The Nef protein is an accessory gene product of HIV and SIV that is dispensable for virus spread in experimental ex vivo cell culture systems. Thus, Nef is an important factor for AIDS pathogenesis. To achieve this multitude of activities, Nef has evolved as versatile adaptor for protein interactions that lacks intrinsic enzymatic activity, which allows the viral protein to affect a wide range of host cell protein sorting and signal transduction processes. We thus chose a strategy aimed at wrapping the surface of Nef by the combination of different, physically linked, target domains and the iterative optimization of domain composition and linker segments.

Mutation of the RT-loop sequence E88AIHHE to VSWSPD (‘NI1-2’) or YSPFSW (‘NI1-3’) led to an increase of the Nef binding affinity to 179 nM or even 48 nM, respectively, indicating the enormous contribution of this region to the PxxPxR recognition of the SH3 domain. In addition, two long antiparallel helices α4 and α5 (residues Y85-K98 and Q108–Q122) of Nef form a characteristic hydrophobic interface for interactions. The accessible surface of helices α4 and α5 is separated into two parts by the highly conserved residues F94 and W117, whose aromatic side chains oppose each other and act as gatekeepers to form a barrier in the helical region. The mutant residues V90SWSPD of the Hck RT loop undergo tight interactions with the proximal region of these antiparallel helices, with tryptophan 92 of Hck contributing itself to the high binding affinity with 41 interactions to six different residues of Nef within a shell of 4 Å. Many of these interactions were mediated by stacking of the aromatic side chains W92Hck to F94Nef, as well as facing interactions to W117Nef. In addition, R81Nef in the PxxPxR motif of Nef showed direct ionic interactions to D96 of Hck and the side chain of Q122Nef made tight interactions to the hydroxyl group of Y89Hck (2.6 Å) and the main chain oxygen of V90Hck (2.9 Å). Likewise, the hydroxyl group of S93Hck was hydrogen bonded to D90Nef (2.6 Å) and D95Hck formed an ionic interaction to K86 of Nef. The 8-fold increase in affinity of the Hck-SH3 RT-loop mutant VSWSPD compared to the EAIHHE wild type sequence is largely due to multiple interactions mediated by the central tryptophane residue. While the site proximal to the PxxP motif harbors the central residues of the RT loop, the distal site covers a newly identified N-terminal helix of Nef (residues 60 to 69) with W61 mediating multiple interactions to hydrophobic residues L104, I113 and L114. Of note, the acidic cluster motif of four successive glutamates (E66–E69), that was reported to interact with the sorting adaptor protein PACS1, adopts a helical conformation on this structure element.

>GAMASSNTAATNADSAWLEAQEEEEVGFPVRPQVPLRPMTYKAALDISHFLKEKGGLEGLIWSQRRQEILDLWIYHTQGYFPDWQNYTPGPGIRYPLTFGWCFKLVPVEPEKVEEANEGENNSLLHPMSLHGMEDAEKEVLVWRFDSKLAFHHMARELHPEYYKDA[2x];>MEDIIVVALYDYVSWSPDDLSFQKGDQMVVLEESGEWWKARSLATRKEGYIPSNYVARVDS[2x]>MASMTGGQQMGRGSAGVLPAHGTQHGIRLPLRSGLGGAPLGLRLPRETDEEPEEPGRRGSFVEMVDNLRGKSGQGYYVEMTVGSPPQTLNILVDTGSSNFAVGAAPHPFLHRYYQRQLSSTYRDLRKGVYVPYTQGKWEGELGTDLVSIPHGPNVTVRANIAAITESDKFFINGSNWEGILGLAYAEIARPDDSLEPFFDSLVKQTHVPNLFSLQLCGAGFPLNQSEVLASVGGSMIIGGIDHSLYTGSLWYTPIRREWYYEVIIVRVEINGQDLKMDCKEYNYDKSIVDSGTTNLRLPKKVFEAAVKSIKAASSTEKFPDGFWLGEQLVCWQAGTTPWNIFPVISLYLMGEVTNQSFRITILPQQYLRPVEDVATSQDD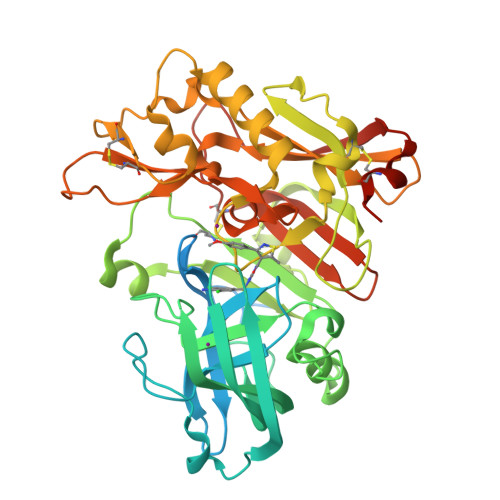CYKFAISQSSTGTVMGAVIMEGFYVVFDRARKRIGFAVSACHVHDEFRTAAVEGPFVTLDMEDCGYNIPQTDEST[4x]>[2x]LAKLYKVSNGAGTMSVSLVADE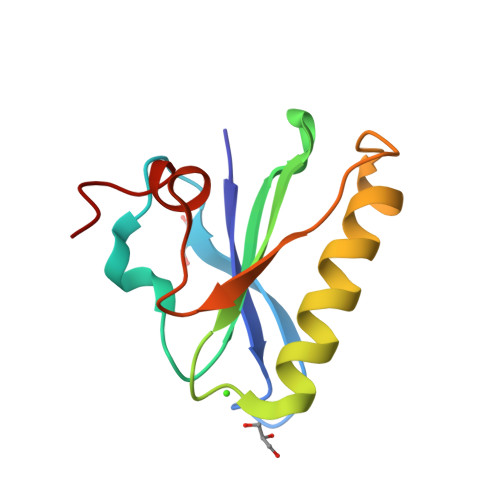NPFAQGALKSEDCFILDHGKDGKIFVWKGKQANTEERKAALKTASDFITKMDYPKQTQVSVLPEGGETPLFKQFFKNWR The Ets transcription factor family consists of 28 genes in humans containing the evolutionarily conserved 85 amino acid Ets DNA-binding domain, originally identified as a viral oncogene (E26 transformation-specific). The Ets domain is a variant helix-turn-helix (winged helix) structure, comprising three α-helices and a four-stranded antiparallel β-sheet. Here, we present the crystal structures of the Ets domains of the entire PEA3 subfamily (Etv1, Etv4, and Etv5) together with the structure of the Erg family member (Fev). Furthermore, a new Ets dimerization interface linked by a redox-sensitive disulfide bond is identified, and this dimerization is shown to result in a significant inhibition of DNA binding, potentially linking Ets transcription factors with cellular redox regulatory mechanisms.

Etv4 and Etv5 DNA complexes were crystallized using oligonucleotide duplexes that had nine complementary base pairs (containing the same consensus sequence) with a single overhanging nucleotide on each end, which makes favorable interactions with neighboring DNA molecules. In all the DNA complex crystals, base pair stacking interactions between neighboring molecules allow the DNA to form a pseudo-contiguous helix that, in some cases, runs the entire length of the crystal. In all four DNA complexes, the recognition helix (α3) inserts deep into the major groove and provides multiple contacts with the base pairs of the core GGAA sequence, as well as with the phosphate backbone. A comparison of the structures of Etv1, Etv4, and Fev in the presence and absence of DNA allows us to identify conformational changes that may occur upon DNA binding. In Etv4, in addition to three residues Arg-397, Arg-400, and Tyr-401 adopting different rotamers, the C-terminal end of the recognition helix switches from a 310 hydrogen bonding pattern (which is the form adopted in all the other ETS structures) to a more canonical α-helical hydrogen bonding pattern, although in this case the difference may be due to the fact an ethylene glycol molecule is bound in the vicinity. Analysis of the contacts between adjacent molecules in the Etv1, Etv4, and Etv5 crystals reveals a conserved potential dimer interface that is distant from the DNA binding surface and is present in all the DNA-free and DNA-bound crystal forms. Dimerization of Etv1, -4, and -5 is mediated by the homologous cysteine residues (Cys-416, Cys-422, and Cys-449, respectively). Similarly, dimeric Etv4 and Etv5 also bind DNA with affinities that are 2 orders of magnitude lower than the reduced monomeric forms (note that the Kd values of the dimeric forms are rough estimates, as saturation could not be reached). DNA complexes of dimeric Etv4 and Etv5 migrate at a lower mobility than complexes of the monomeric proteins, indicating the presence of a dimer of Etv4/5 with one or two bound probe molecules.

>SMRGALQLWQFLVALLDDPTNAHFIAWTGRGMEFKLIEPEEVARLWGIQKNRPAMNYDKLSRSLRYYYEKGIMQKVAGERYVYKFVCEPDALFSMAFPDN[8x]>MIEKDVVQILKAVSEFYPGRFQPDDLKGTVKAWHRVLAEYELEEIMNNLTDYAKVNKFPPTVSDLLKAQSEQRDRFIPSYEETQRILKEQAEAEEAARNDPDLQAAQEENMRKIREMLGI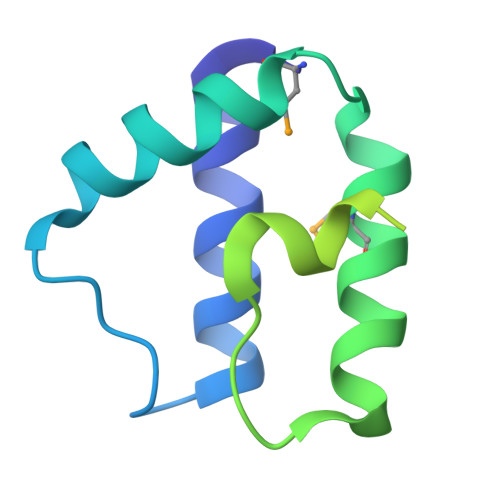NRGGAR[3x]5-hydroxy,-4,5-dihydroquinolinate | C7 H7 N O5 | 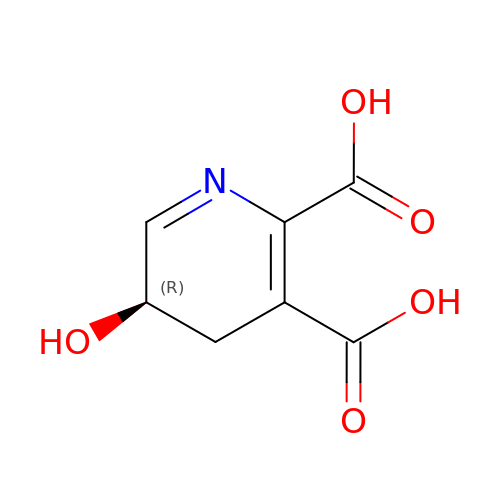DNLLCWBTFPFCLN-GSVOUGTGSA-N~{N}4-[(4-fluorophenyl)methyl]-6-(trifluoromethyl)pyridine-2,4-diamine 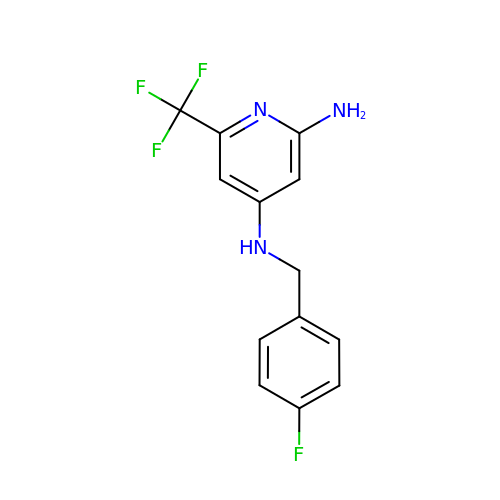| C13 H11 F4 N3 | NVURBNAAKDVJHE-UHFFFAOYSA-N> FQGMLPRDERRGQLLVVASDVFVDRGYHAAGMDEIADRAGVSKPVLYQHFSSKLELYLAVLHRHVENLVSGVHQALSTTTDNRQRLHVAVQAFFDFIEHDSQGYRLIFENDFVTEPEVAAQVRVATESCIDAVFALISADSGLDPHRARMIAVGLVGMSVDCARYWLDADKPISKSDAVEGTVQFAWGGLSHVPL

We had previously identified the transcription factor FasR, as a key activator of fas and acpS gene expression. fas and acpS, respectively, coding for FAS I synthase and 4-phosphopantetheinyl transferase (essential to produce functional ACP), form a single operon in Mtb. FasR:DNA binding is regulated by long-chain acyl-CoAs, which are themselves products of FAS I, namely acyl-CoAs ≥ C16 disrupt the interaction of Mtb FasR with its cognate DNA6. FasR is a TFR member that senses long and very long acyl-CoA moieties, subsequently turning off FAS I-mediated fatty acid biosynthesis. We have now determined the 3D structures of FasR from Mtb, in three different states obtained with the protein (i) crystallised alone, (ii) co-crystallised in complex with the fatty acid C20-acyl-CoA and (iii) in complex with a double-stranded DNA oligonucleotide bearing the specific FasR-binding sequence.

FasRΔ33 readily crystallised in the absence of added ligands and also in complex with acyl C20-CoA (arachinoyl- or arachidoyl-CoA). The FasRΔ33-C20-CoA dimer is strictly symmetric, with the crystallographic twofold axis relating one protomer to the other. A striking feature of FasRΔ33-C20-CoA is a tunnel-like cavity, delimited by helices α4, α5, α7 and α8, with its two openings towards the bottom and the top of the EBD. C20-CoA binds within this tunnel, in a parallel orientation with respect to core helices α4, α5 and α7. The tunnel is ~28 Å long, with a predominance of hydrophobic residues on its wall pointing their side chains towards the lumen of the tunnel. Towards the cavity’s upper entrance, most of the 4′-phosphopantetheine portion of the CoA cofactor is also observed, the sulfur atom (due to its stronger electron density) was instrumental in positioning the whole C20-CoA moiety. Electron density becomes less clear towards the tip of the pantoic group, likely due to high mobility of the CoA portion, eventually vanishing in the region corresponding to the 3′-phosphoadenosine diphosphate group, which were thus not included in the final model. In FasRΔ33-C20-CoA, the dimer is opened up, with both protomers separating away from each other, compared with FasRΔ33-C14. Using the position of conserved Tyr77 Cα as a reference (at the centre of helix α3, key to mediate DNA-binding), the two HTH domains in FasRΔ33-C14 are ~48 Å apart, vs ~57 Å in FasRΔ33-C20-CoA. Taking the above observations together, we hypothesize that binding of a ligand, long enough to fill up the entire hydrophobic tunnel, stabilises the FasR dimer in a more rigid configuration, fixing an open HTH geometry that is incompatible to bind DNA. A fully extended C20 acyl chain measures 26.5 Å, within the FasR-C20-CoA tunnel the acyl shows some bending reducing that length to ~20 Å. The latter magnitude is enough for the C20 chain to fully occupy the tunnel, its distal tip located immediately beside the bottom opening that leads to the space between protomers in the dimer.>[2x]MSQHNILEALNVRVVGTGDRILFLAHGFGTDQSAWHLILPYFTQNYRVVLYDLVCAGSVNPDYFDFNRYTTLDPYVDDLLNIVDSLGIQNCAYVGHSVSAMIGIIASIRRPELFSKLILIGFSPRFLNDEDYHGGFEEGEIEKVFSAMEANYEAWVHGFAPLAVGADVPAAVREFSRTLFNMRPDISLFVSRTVFNSDLRGVLGLVRVPTCVIQTAKDVSVPASVA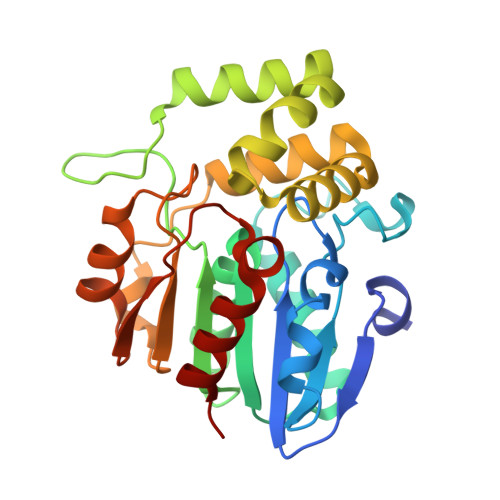EYLRSHLGGDTTVETLKTEGHLPQLSAPAQLAQFLRRALPR> AEQATKSVLFVCLGNICRSPIAEAVFRKLVTDQNISENWRVD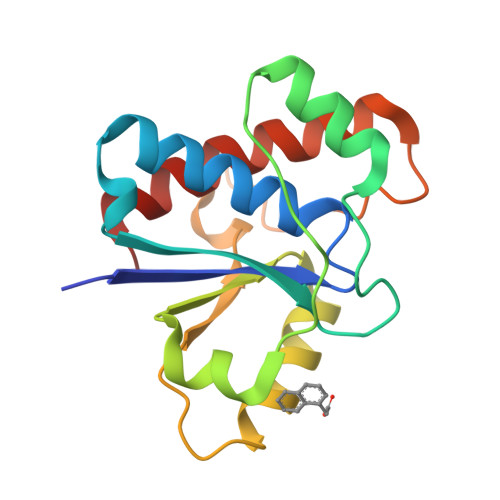SAATSGYEIGNPPDYRGQSCMKRHGIPMSHVARQITKEDFATFDYILCMDESNLRDLNRKSNQVKTCKAKIELLGSYDPQKQLIIEDPYYGNDSDFETVYQQCVRCCRAFLEKAH> SLSEAGYPRKVMQHAEELHERILSFDSRITVPLDFGTTGNEVDKDGPGQLDLVKAGRGRLSGAALAIFGWPEMWNGPNAPHKPTPGFVDEARHQQEIRYKILTGMVRDFPNQVGIAYSPEDFRRLAMEGKFAIVMSMLN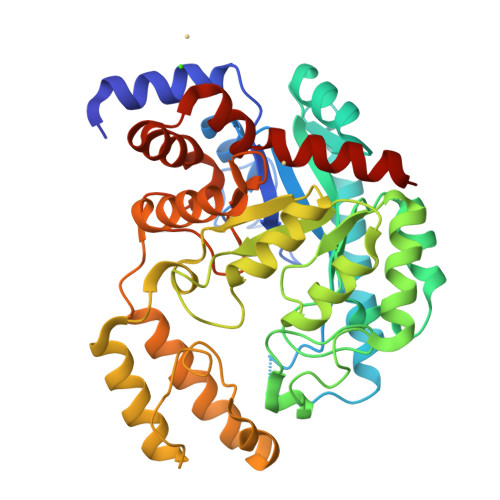AYPLGDDLSQLDKWAARGVRMFGFSYVGNNDWADSSRPLPFFNDSPDALGGLSPLGKQAVERLNDLGVIIDVSQMSTKALEQVAALSRAPIVASHSAPRALVDIKRNLSDHEMQLIKDSGGVIQVVGFPAYLRPLSKPTLDKLDALRARFDLPPLEGLDYALMPGDPIITIWPEQRFGEYASALYGILEEEPKAGLKELVDAIDYTVKKVGIDHVGISSDFNDGGGVDGWKDVSEIRNVTAELITRGYSDADIAKLWGGNFLRAWGEVQKRAKPTATP> EDKRAKVTSAMQTMLFTMLRKLDNDALNNIINNARDGCVPLNIIPLTTAAKLMVVIPDYNTYKNTCDG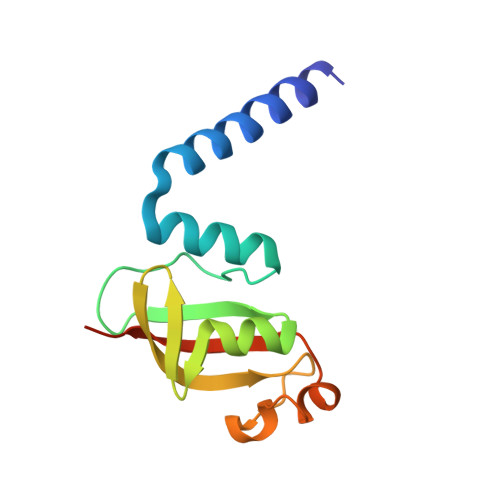TTFTYASALWEIQQVVDADSKIVQLSEISMDNSPNLAWPLIVTALRANSAVKLQ>[2x]MGKVRNISGCVAVAHGVRLADVDVICSYPIRPYTGIMSELARMVADGELDAEFVHGEGEHAQLSVVYGASAAGARVFTGSSGVGVTYAME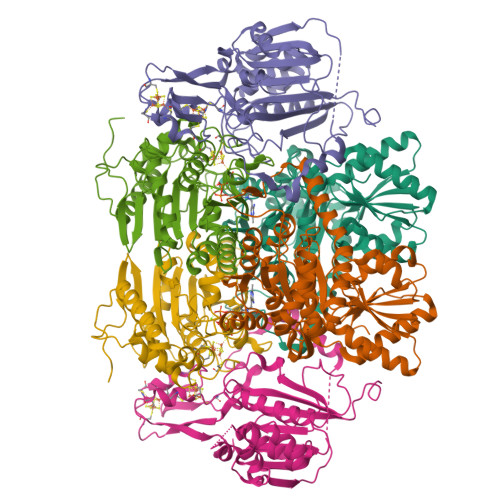VYSPISGERLPVQMAIADRTLDPPGDFGEEHTDAECCRDQGWIQGWASTPQEALDNTLIYYRVGEDQRVLLPQYACLDGYFVSHILGPVDIPDEAQVKEFLPPYKNHHVLDPRKPQIIGPQIEPAMGPPLQYQRYQAVKGVHKVLEEACDEFARIFGRKYDPYLDEYLTDDAEVIIFGQGAHMETAKAVARRLRNLGEKVGVARLRTFRPFPTEQIKERLSKFKAIGVLDVSANFGISCSGGVLLSELRAALYDYGDKVKTVGFVAGLGGEVVTHDEFYRMFQKLKEIAKTGKVEQTSYWIPFEL;>MSTKDLFAEPNLKQITVWARGVVMNKDARDIVVALTEAAAKEGKYVQAWENYVDLPDRIYVPVRAYARISSDPIESKYIYENETPDIVVLVEESLIKGVPILKGIRPGSTLVVNTKRSIDTILEFLGDTGNLAQIVTVDANSMAEAVMTLSGAEGATDATGIGAGIAAPIAGAVVKATGIVDVENLAAVVKNPAAMRRGYAEAQVRQLPPHEAVEEAAVSATELLRQMPFAGTVPSPVTENEGMVTGNWRIQRPIIDREACTECYTCWIYCPDSCITRTEEGPVFNMKYCKGCGLCTAVCPSGALTNVPELDFKD[2x];>[2x]MLDRIASIKKAPDEEYYVPGHRTCAGCGPALTYRLVAKAAGPNTIFIGPTGCMYVANTSYGCGPWRVPWIHAQITNGGAVASGIEAAYKAMIRKKKTDAEFPNIIVMAGDGGAVDIGLQALSAMLYRGHDVLFICYDNESYANTGIQTSPTTPYGANTTFTPPGEVVPEGKKLFPKDNPKVIAHGHPELKYVATASIGWPVDLMNKVRKGLNQEGPAYIHIHAPCPKGWQFPADKTIEMAKLAVQTGMFQLYEYENGEYKLSVKVDKRKPVSEYMKLQKRFAHLKPEHIAKMQAFVDARCAEVGITVPVVASNA> AITKPLLAATLENIED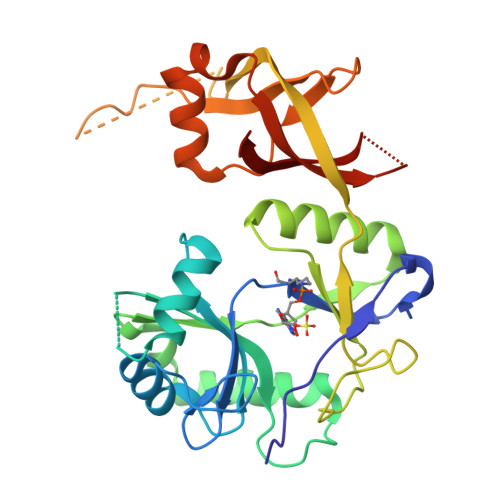VQFPCLATPKIAGIRSVKQTQMLSRTFKPIRNSVMNRLLTELLPEGSDGEISIEGATFQDTTSAVMTGHKMYNAKFSYYWFDYVTDDPLKKYIDRVEDMKNYITVHPHILEHAQVKIIPLIPVEINNITELLQYERDVLSKGFEGVMIRKPDGKYKFGRSTLKEGILLKMKQFKDAEATIISMTALFKNTNTKTKDNFGYSKRSTHKSGKVEEDVMGSIEVDYDGVVFSIGTGFDADQRRDFWQNKESYIGKMVKFKYFEMGSKDCPRFPVFIGIRHEEDR> MPVHGVIYYSSPSMATFLSPAQDNLVRTYFAQHLKKWVVQYKLYRNAVTPKTLEFLKQNINPSMLACVDE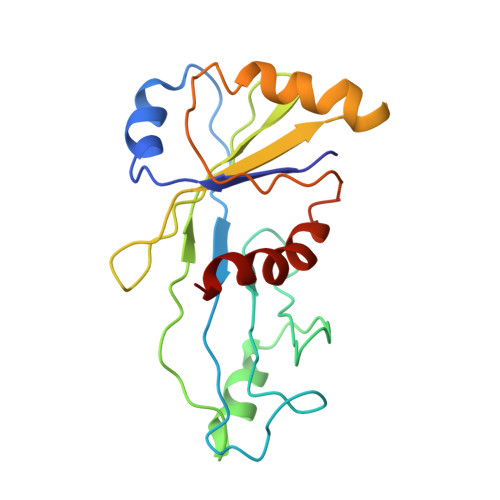ATMIDAEPELEDIIVRTKLWNFRQSFTIEGSIYEVGSFKVAIANVLQKSVWKGILFHVTYDGTESVDLARPIIQEFFLKCFLQNNKSVTPVYESFFNQPRHSLDSKLLLQLFKQRIDTVSQRT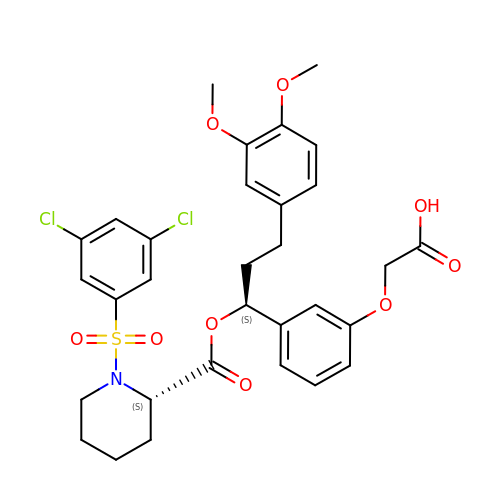{3-[(1S)-1-[({(2S)-1-[(3,5-dichlorophenyl)sulfonyl]piperidin-2-yl}carbonyl)oxy]-3-(3,4-dimethoxyphenyl)propyl]phenoxy}acetic acid | C31 H33 Cl2 N O9 S | AOMAGJKZRYWVSR-SVBPBHIXSA-N> MKYMITSKGDEKSDLLRLNMIAGFGEYDMEYDDVEPEIVISIGGDGTFLSAFHQYEERLDEIAFIGIHTGHLGFYADWRPAEADKLVK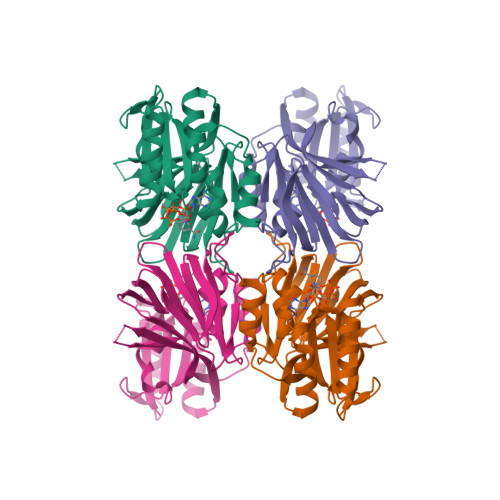LLAKGEYQKSSYPLLKTTVKYGIGKKEATYLALNESTVKSSGGPFVVDVVINDIHFERFRGDGLCMSTPSGTTAYNKSLGGALMHPSIEAMQLTEMASINNRVYRTIGSPLVFPKHHVVSLQPVNDKDFQISVDHLSILHRDVQEIRYEVSAKKIHFARFRSFPFWRRVHDSFIEDLEHHHHHH>MVLVLDFGSQYTRLIARRLRELRAFSLILPGDAPLEEVLKHRPQALILSGGPRSVFDPDAPRPDPRLFSSGLPLLGICYGMQLLAQELGGRVERAGRAEYGKALLTRHEGPLFRGLEGEVQVWMSHQDAVTAPPPGWRVVAETEENPVAAIASPDGRAYGVQFHPEVAHTPKGMQILENFLELAGVKRDWTPEHVLEELLREVRERAGKDRVLLAVSGGVDSSTLALLLAKAGVDHLAVFVDHGLLRLGEREEVEGALRALGVNLLVVDAKERFLKALKGVEDPEEKRKIIGREFVAAFSQVARERGPFRFLAQGTLYPDVIESAGGHGAAKIKSHHNVGGLPEDLEFELLEPFRLLFKDEVRELALLLGLPDTLRLRHPFPGPGLAVRVLGEVTEERLEILRRADDIFTSLLREWGLYEKVAQALAVLTPVRSVGVAGDERKYGYVLALRAVTTEDFMTADWARLPL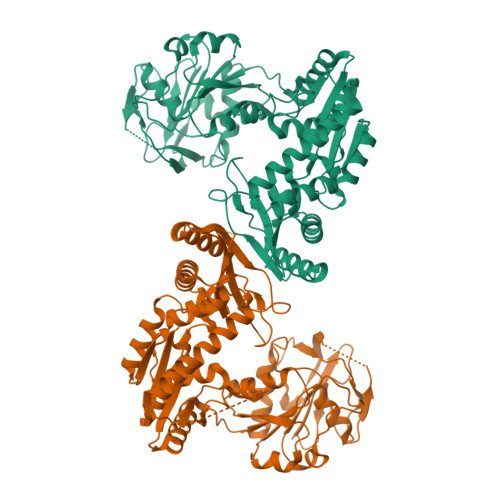EFLDEAARRITRRVPEIGRVVYDLTSKPPATIEWE[4x]>MSESPMFAANGMPKVNQGAEEDVRILGYDPLASPALLQVQIPATPTSLETAKRGRREAIDIITGKDDRVLVIVGPCSIHDLEAAQEYALRLKKLSDELKGDLSIIMRAYLEKPRTTVGWKGLINDPDVNNTFNINKGLQSARQLFVNLTNIGLPIGSEMLDTISPQYLADLVSFGAIGARTTESQLHRELASGLSFPVGFKNGTDGTLNVAVDACQAAAHSHHFMGVTKHGVAAITTTKGNEHCFVILRGGKKGTNYDAKSVAEAKAQLPAGSNGLMIDYSHGNSNKDFRNQPKVNDVVCEQIANGENAITGVMIESNINEGNQGIPAEGKAGLKYGVSITDA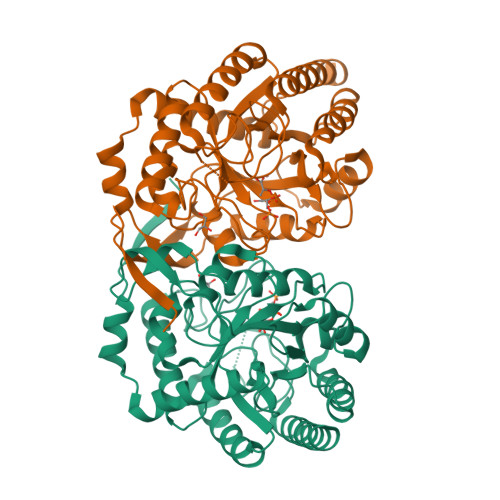CIGWETTEDVLRKLAAAVRQRREVNKK[2x]The three largest gene segments of the Thogotoviruses, THOV, DHOV and JOSV are homologous to those of IAV and code for the heterotrimeric polymerase. In this paper we present the atomic structures of the putative PB2 cap binding and 627 domains of THOV and the putative PA N-terminal endonuclease domains of THOV and DHOV. Despite very low sequence homologies, all domains have similar folds to those of the corresponding IAV polymerase domains. However, the critical active site residues in the putative cap binding and endonuclease domains are not conserved in THOV and DHOV and, contrary to the case of IAV polymerase, neither domain shows the expected in vitro biochemical activity.

The corresponding construct (residues 1 to 169) was cloned, expressed, purified and crystallized. The structure could not be solved by molecular replacement using that of IAV PA-Nter due to low sequence homology. THOV PA-Nter comprises four principle β-strands surrounded by six α-helices. Comparison of the two independent molecules in the asymmetric unit of crystal form 1 shows that the region 72–89, including helix α3 and the following loop, is in two very distinct orientations. In chain A, this element is positioned as in DHOV and IAV (see below) whereas in chain B it is dissociated from the body of the protein, rotated by 90° and inserted between two neighbouring molecules in the crystal. For THOV and DHOV PA-Nter the putative active site is more like an extended groove and furthermore, is positively charged. The extra positive charge in the putative active sites of THOV and DHOV PA-Nter arises from the replacement of acidic residues and the introduction of extra lysines (Lys38, Lys61 and Lys97 for THOV and Lys39 and Lys100 for DHOV PA-Nter). Surprisingly, for the THOV domain, addition of Mn2+ or Mg2+ ions destabilises the protein by 3–6°C. Interestingly, the significant difference in thermal stability behaviour of the THOV and DHOV domains correlates with the enhanced plasticity and much poorer diffracting crystals of THOV PA-Nter.

>[2x]GMGSGMAMTDRPDHIDSRVWELSETQEDWITQVHGHVRRVVECWKYTICCLISNMHTHRGAPQYDVFKWQDRSTIEWICSKKKVQYPERDTPDLYDNERAVAYKVLLVSDLSDHSPTSGIYHDLAFNLEGEAEESCALVLRGSQLQDIKGFLCRALEWVVSNNLTQEVVETISGEAK> VTYPGAIPLSLTSNYETPSPTAIPLEPTPTATGTAELDALWNLVEAQYPVQTAAVTTLVTVPDDYKFEADPPSYALAGYETSEIAGLKFPKGFKFGVAGAAIQVEGAAKAEGRGPSTWDYLCHHYASTQCNNYDPDITTNHYYLYPLDFARLQHLGINTYSFSISWTRIYPLGAGYVNEAGLAHYDAVIHSAKKYGLEPVGTVFHWDTPLSLMLKYGAWQDTGDQIVKDFVTYATTVFKRYGNEVKTWFTFNEPRVFCSQNSGLPYNLTYPEGINSTSAVFRCTYNVLKAHGHAVKVYRDLVASGTIAAGEI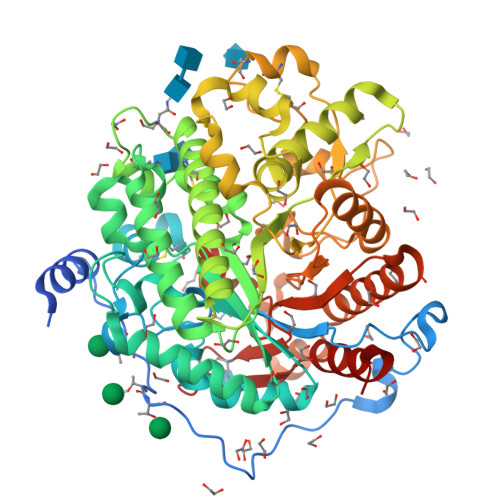GFKSDDNYPIPARPGNADDEESAKRHEAFRIGIFAQPVYGNGDYPDVVKETVGDMLPALTDEDKGYIKGSGDIFAIDGYRTDISHAALNGIANCIRNQSDPNWPVCEEGSDPFAHVYPSGFAIGQSADPLSSWLVNSAPFIRDQLKFLTQTYPAKGGIYFSEFGWAEDAEYDRQLLYQITWDGLRTQYLTDYLSQLLLAVHKDGINLRGALTWSFVDNWEWGLGMQQKFGFQFVNQSDPDLTRTFKLSAHAYAQFGRNHLHHHHHH>[2x]GHMFQCNVPLGMESGRIANEQISASSTYSDGRWTPQQSRLHGDDNGWTPNLDSNKEYLQVDLRFLTMLTAIATQGAISRETQNG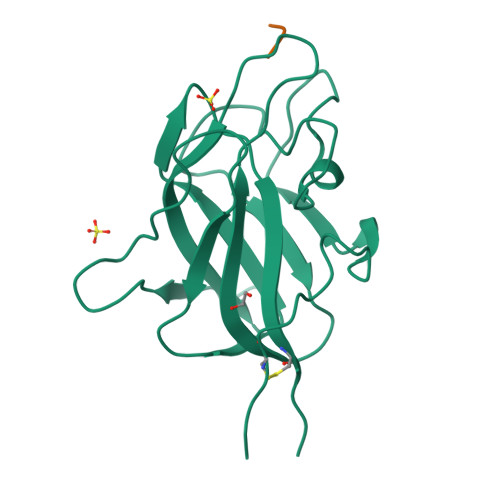YYVKSYKLEVSTNGEDWMVYRHGKNHKVFQANNDATEVVLNKLHAPLLTRFVRIRPQTWHSGIALRLELFGCRVTSGS;>XSIIRR[2x]Curli proteins are produced via dedicated and tightly regulated cellular processes, and their fibrils mediate host cell adhesion and invasion, lead to immune system activation, and scaffold bacterial communities known as biofilms. The two key players in curli fibril formation are CsgA and CsgB, the major and minor curli subunits, respectively. CsgA, a 151-residue protein, consists of five imperfect sequence repeats (R1-R5), defined by regularly spaced serine (Ser), glutamine (Gln) and asparagine (Asn) residues. The first and the last repeats (R1 and R5) form amyloid fibrils in isolation and are critical to CsgA seeding and nucleation by CsgB, while the other repeats (R2-R4) contain 'gatekeeper' residues that temper the amyloidogenicity of CsgA.

However, while 45LNIYQY50 (R1), 47IYQYGG52 (R1), and 137VTQVGF142 (R5) formed unbranched and elongated amyloid-like fibrils, the 129TASNSS134 (R4-R5 loop) segment formed scarce and more amorphous structures. The 45LNIYQY50 (R1), 47IYQYGG52 (R1), and 137VTQVGF142 (R5) segments bound the amyloid indicator dye ThT and demonstrated dose-dependent amyloid fibrillation curves with short lag times. 45LNIYQY50 and 47IYQYGG52, which are overlapping segments from the R1 repeat, adopted very similar structures. Both segments, as well as 137VTQVGF142 (R5), adopted a classical amyloid steric zipper architecture, with two possible dry interfaces between paired β-sheets. The β-strands were oriented parallel to each other along the β-sheets. These three structures are class 1 steric zippers, as defined by Sawaya and Eisenberg according to the organization of the β-strands and β-sheets. In each of these dry interfaces, the chemical properties governing fibril stability, i.e., buried surface area and shape complementarity between sheets, resembled those of eukaryotic steric zipper structures. Specifically, the R1 45LNIYQY50 and 47IYQYGG52 segments and the R5 137VTQVGF142 segment formed fibrils that bound the amyloid indicator dye ThT and formed canonical amyloid class 1 steric zippers. These segments contain Gln49 or Gln139 (marked in bold in 45LNIYQY50, 47IYQYGG52, and 137VTQVGF142), which are critical for fibrillation and cannot be mutated to asparagine without interfering with curli assembly. The R1 segment 47IYQYGG52 and the control segment 129TASNSS134 showed a milder effect on the fibrillation rate of Aβ1–40.

> IYQYGG>[2x]GNKWNTTLPGGNMQFQGVIIAETCRIEAGDKQMTVNMGQISSNRFHAVGEDSAPVPFVIHLRECSTVVSERVGVAFHGVADGKNPDVLSVGEGPGIATNIGVALFDDEGNLVPINRPPANWKRLYSGSTSLHFIAKYRATGRRVTGGIANAQAWFSLTYQ;> MGVALGATRVIYPAGQKQEQLAVTNNDENSTYLIQSWVENADGVKDGRFIVTPPLFAMKGKKENTLRILDATNNQLPQDRESLFWMNVKAIPSMDKSKLTENTLQLAIISRIKLYYRPAKLALPPDQAAEKLRFRRSANSLTLINPTPYYLTVTELNAGTRVLENALVPPMGESTVKLPSDAGSNITYRTINDYGALTPKMTGVMEHHHHHH;> DLYFNPRFLADDPQAVADLSRFENGQELPPGTYRVDIYLNNGYMATRDVTFNTGDSEQGIVPCLTRAQLASMGLNTASVAGMNLLADDACVPLTTMVQDATAHLDVGQQRLNLTIPQAFMSNRARGYIPPELWDPGINAGLLNYNFSGNSVQNRIGGNSHYAYLNLQSGLNIGAWRLRDNTTWSYNSSDRSSGSKNKWQHINTWLERDIIPLRSRLTLGDGYTQGDIFDGINFRGAQLASDDNMLPDSQRGFAPVIHGIARGTAQVTIKQNGYDIYNSTVPPGPFTINDIYAAGNSGDLQVTIKEADGSTQIFTVPYSSVPLLQREGHTRYS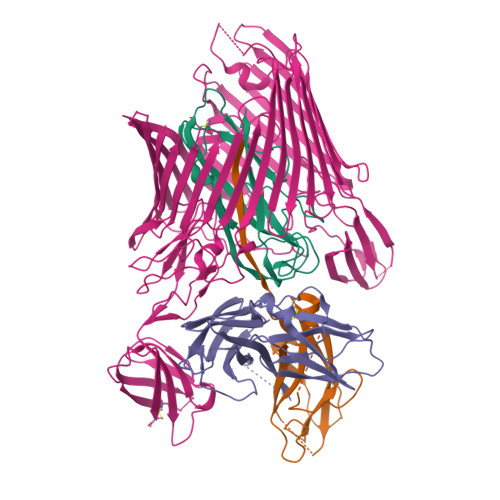ITAGEYRSGNAQQEKPRFFQSTLLHGLPAGWTIYGGTQLADRYRAFNFGIGKNMGALGALSVDMTQANSTLPDDSQHDGQSVRFLYNKSLNESGTNIQLVGYRYSTSGYFNFADTTYSRMNGYNIETQDGVIQVKPKFTDYYNLAYNKRGKLQLTVTQQLGRTSTLYLSGSHQTYWGTSNVDEQFQAGLNTAFEDINWTLSYSLTKNAWQKGRDQMLALNVNIPFSHWLRSDSKSQWRHASASYSMSHDLNGRMTNLAGVYGTLLEDNNLSYSVQTGYAGGGDGNSGSTGYATLNYRGGYGNANIGYSHSDDIKQLYYGVSGGVLAHANGVTLGQPLNDTVVLVKAPGAKDAKVENQTGVRTDWRGYAVLPYATEYRENRVALDTNTLADNVDLDNAVANVVPTRGAIVRAEFKARVGIKLLMTLTHNNKPLPFGAMVTSESSQSSGIVADNGQVYLSGMPLAGKVQVKWGEEENAHCVANYQLPPESQQQLLTQLSAECRLVPRGSWSHPQFEK>MGHHHHHHMKSLRETESWKLLESSIIYYEGNPIGTVAAQDPELAALNYDQCFLRDFVPSAFVFLMDGQTDIVRNFLIETLTLQSHEKEMDCFQPGAGLMPASFKVESDGSKEYLVADFGEKAIARVPPVDSCMWWILLLRAYEKATGDLTLAREPKFQAGIKLILDLCLAHRFSMYPTMLVPDGAFMIDRRMGVYEHPLEIQVLFYAALRAARELLLPDGDGEQYLNKVHGRLGALQYHIRNYYWVDLKRLREIYRYKGNEFGKEIANKFNIFSQSIPDWVIEWLPEKGGYLAGNLGPGRMDFRFFALGNLMAILAGLASEEESQRIMNLFAHRWEDLIGYMPVKICYPALQGLEWQIVTGCDPKNIPWSYHNGGNWPVLLWLFTAAALKTGKVELAHEAIA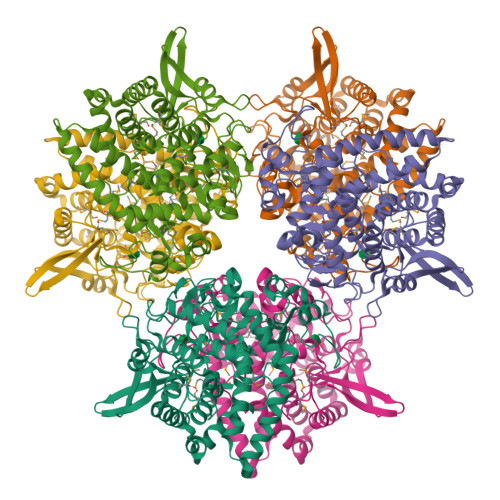IAEGRLSNDKFPEYYDGNNGRLIGKEARIYQTWSIAGLLVAKQFLANPDHVEFISFPDT[3x]> QPSRKEKSLGLLCHKFLARYPNYPNPAVNNDICLDEVAEELNVERRRIYDIVNVLESLHMVSRLAKNRYTWHGRHNLNKTLGTLKSIGEENKYAEQIMMIKKKEYEQEFDFIKSYSIEDHIIKSNTGPNGHPDMCFVELPGVEFRAASVNSRKDKSLRVMSQKFVMLFLVSTPQIVSLEVAAKILIGEDHVEDLDKSKFKTKIRRLYDIANVLSSLDLIKKVHVTEERGRKP

Whereas the E2F proteins 1–6 bind to DNA preferentially as heterodimers with the related DP proteins DP1 and DP2, the two most recently discovered members of the E2F family, E2F7 and E2F8, are ‘atypical‘, because they contain two distinct DNA-binding subdomains. They also lack the pocket protein-binding domain found in all other E2Fs, and thus are not regulated by the canonical cyclin-dependent kinase/retinoblastoma protein pathway. In this work, we have determined the three-dimensional structure of a non-canonical E2F, E2F8, bound to its preferred DNA sequence. In summary, through extensive structural and functional analyses of the E2F proteins, we have defined the DNA-binding specificities of E2F and E2F/DP complexes. These analyses have revealed that the two domains of the atypical repressor E2Fs correspond to the E2F and DP domains, which bind to DNA sites that are indistinguishable from those bound by typical E2F/DP heterodimers.

Analysis of the structure derived from a cubic and hexagonal crystal forms revealed that both DBDs are composed of three α-helixes and a small antiparallel β-sheet. However, the comparison of E2F8's first and second DBDs to E2F4 and DP2, respectively, revealed striking structural similarity between them (r.m.s.d.=2.7 and 1.9 Å, respectively), despite the sequence identity being only 39.7 and 27.5%. The E2F8 DBDs 1 and 2 are thus referred to as DBDE2F and DBDDP hereafter. Of the 82 residues that comprise the linker, 23 are resolved in the structure, forming two α-helixes that wrap around the surface of the DBDE2F and DBDDP on the opposite side of the bound DNA. Whereas the interaction between typical E2Fs and DP proteins is mediated by separate interaction domains, in E2F8, the linker between the DBDs strongly contributes to the inter-DBD interaction. The two DBDs of E2F8 recognize a 5′-GGCGGG-3′ core sequence by inserting their helices α3 into the same major groove of DNA. The preference to the 5′ and 3′ flanking sequences is due to contacts formed by Arg113, Lys114 and Ser117, and Lys175 in the minor grooves, respectively. The major difference between the structures is that in contrast to E2F4/DP2, E2F8 binding to DNA is not symmetrical, due to differences between DNA recognition by DP2 and the E2F8 DP domain. The first Arg residue 313 of this motif in E2F8 DBDDP forms specific contacts with the oxygen atom of guanine G10′. We also observed an interaction between symmetry-related molecules that involved helix α1 that potentially facilitates the dimerization of two E2F8 proteins.Glycan uptake across the bacterial outer membrane (OM) of these bacteria is mediated by SusCD protein complexes, comprising a membrane-embedded barrel and a lipoprotein lid, that is thought to open and close to facilitate substrate binding and transport. Here we show that for both the levan and dextran utilisation systems of Bacteroides thetaiotaomicron, the additional OM components assemble on the core SusCD transporter, forming stable glycan utilising machines which we term ‘utilisomes’. Transport-competent FOS are generated from levan by a surface-exposed lipoprotein, a GH32-family levan endo-glycanase (GHlev), while an SGBP (SGBPlev) is thought to recruit levan at the cell surface. Single particle cryogenic electron microscopy (cryoEM) structures in the absence and presence of substrate reveal concerted conformational changes that demonstrate the mechanism of substrate capture, and rationalise the role of each component in the utilisome.

Subsequent 3D classification revealed ~52 % of the particles contain a SusCDlev core transporter, as well as two copies of both GHlev and SGBPlev. We propose that this octameric complex with two copies of each of the four components represents the complete levan utilisome. The structure of the apo levan utilisome was initially assessed using 3D classification. We identified two regions of conformational heterogeneity: the C-terminal domain of SGBPlev, and in the position of the SusDlev lids (ED Fig. 4a-d). Despite the conformational heterogeneity in the position of the SusDlev lid, SusClev, GHlev, and the N-terminal domain of SGBPlev constitute a rigid unit with two-fold (C2) symmetry. Application of a mask that excluded the density for the SusDlev lids followed by focused refinement allowed inclusion of all particles, regardless of SusDlev position, and resulted in a map with a global resolution of 3.5 Å, allowing us to refine models for SusClev and GHlev, and to build de novo the N-terminal domain of SGBPlev. In this substrate-free utilisome structure, there is clear density for only the two N-terminal, Ig-like domains with the second being weaker than the first. Poorly-resolved density is present for the C-terminal, levan-binding domain which extends away from the transporter, towards the extracellular space, with diffuse density visible only at high threshold levels.

>[2x]MPGIMKNKKLLCSVCFLFAFMSALWGQNITVKGNVTSKTDGQPIIGASVVETTATTNGTITDFDGNFTLSVPVNSTLKITYIGYKPVTVKAAAIVNVLLEEDTQMVDEVVVTGYTTQRKADLTGAVSVVKVDEIQKQGENNPVKALQGRVPGMNITADGNPSGSATVRIRGIGTLNNNDPLYIIDGVPTKAGMHELNGNDIESIQVLKDAASASIYGSRAANGVIIITTKQGKKGQIKINFDASVSASMYQSKMNVLNTEQYGRAMWQAYVNDGENPNGNALGYAYNWGYNADGNPVLYGMTLSKYLDSKNTMPVADTDWFDEITRTGVIQQYNLSVSNGSEKGSSFFSLGYYKNLGVIKDTDFDRFSARMNSDYKLIDDILTIGQHFTLNRTSEVQAPGGIIETALDIPSAIPVYASDGSWGGPVGGWPDRRNPRAVLEYNKDNRYTYWRMFGDAYVNLTPFKGFNLRSTFGLDYANKQARYFTYPYQEGTQTNNGKSAVEAKQEHWTKWMWNAIATYQLEVGKHRGDVMIGMELNREDDSHFSGYKEDFSILTPDYMWPDAGSGTAQAYGAGEGYSLVSFFGKMNYSYADRYLLSLTLRRDGSSRFGKNHRYATFPSVSLGWRITQENFMKELTWLDDLKLRASWGQTGNQEISNLARYTIYAPNYGTTDSFGGQSYGTAYDITGSNGGGVLPSGFKRNQIGNDNIKWETTTQTNVGIDFSLFKQSLYGSLEYYYKKATDILTEMAGVGVLGEGGSRWINSGAMKNQGFEFNLGYRNKTAFGLTYDLNGNISTYRNEILELPETVAANGKFGGNGVKSVVGHTYGAQVGYIADGIFKSQDEVDNHATQEGAAVGRIRYRDIDHNGVIDERDQNWIYDPTPSFSYGLNIYLEYKNFDLTMFWQGVQGVDIISDVKKKSDFWSASNVGFLNKGTRLLNAWSPTNPNSDIPALTRSDTNNEQRVSTYFVENGSFLKLRNIQLGYTVPAVISKKMRMDRLRFYCSAQNLLTIKSKNFTGEDPENPNFSYPIPVNITFGLNIGF;>MMKNMILPIAFTALIASMTACSDETDPILTQKNWDGTATYFQSSDEHGFSMYYKPQVGFVGDPMPFYDPVAKDFKVMYLQDYRPNPEATYHPIFGVATKDGATYESLGELISCGGRDEQDAAIGTGGTIYNPADKLYYTFYTGNKFKPSSDQNAQVVMVATSPDFKTWTKNRTFYLKGDTYGYDKNDFRDPFLFQTEDGVYHMLIATRKNGKGHIAEFTSADLKEWESAGTFMTMMWDRFYECPDVFKMGDWWYLIYSEQASFMRKVQYFKGRTLEDLKATTANDAGIWPDNREGMLDSRAFYAGKTASDGTNRYIWGWCPTRAGNDNGNVGDVEPEWAGNLVAQRLIQHEDGTLTLGVPDAIDRKYTSAQEVKVMAKDGNMIESGKTYTLGEGASVIFNRLKVHNKISFTVKTASNTDRFGISFVRGTDSASWYSIHVNADEGKANFEKDGDDAKYLFDNKFNIPADNEYRVTIYSDQSVCVTYINDQLSFTNRIYQMQKNPWSLCCYKGEITVSDVQVSTY[2x];>MKSIIKQLYTILLVTVACLTVTGCSDDFKSGLRLDGDVWVNSIRLDEYAGTVDYQNKAIVVGVPYDYDITRMVVTEMNLSEGAKASIAIGETIDFSLPVSLTVKNGDVQMSYTITVKRDEAKILTFKLNDTYVGKVDQLSKTISVVVPLTVDITQLKGTFTVTDGATVTPASGSIQDFTNPVTYTATYRSAVTPYVVTVTQGNVIPTAFVGTASSVSLLTSPEEKAAAQWMMDNVSMSEYISFKDVVDGKVDLGKYTAIWWHFHADNGDNPPLPDDAKAAAEKFKVYYQNGGNLLLTRYATFYIANLGIAKDERVPNNSWGGNEDSPEITSAPWSFLITGSESHPLFQDLRWKDGDKSTVYTCDAGYAITNSTAQWHIGTDWGGYDDLNAWRNLTGGIDLAHGGDGAVVIAEFEPRSNSGRTLCIGSGCYDWYGKGVDASADYYHYNVEQMTLNAINYLCK[2x]> MGAAQSVNGVKIVTNAYAEIMTDLAVDQDITADQTQVFSIDNVSGDVYVEGTVMTEKLVINLASLMKAVTNQSSQDELIDNIAQQAQAAVSGLNFAQF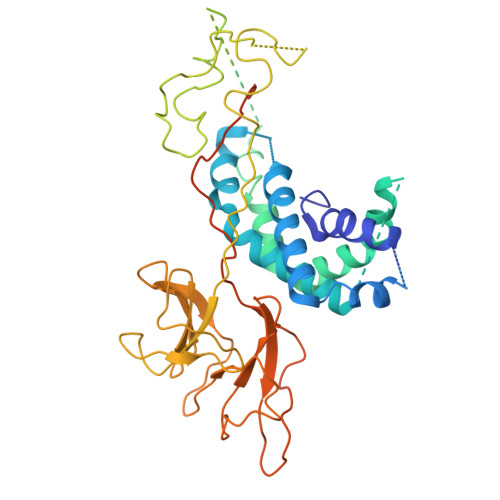AFVTNNIDRLITACVKLSVDMRVSCTAKVEMTQSFSVSSVMGDVRVKDVRMEEFSDVISTCALNAAITNAQLSDIVSQIKQRGDATATGLNPMAILAAVVLAIIGLPLGAGFLAGRRVVGPLMMVTGMVGGGALAMGYVPEPIKLTGFAPEPDLTAVVPVAVENGLTLKAAISKLTGDPQYGAVYWQNYKVTGTTAVKLNQTVSYYAPPNFDPVTWTASEPAQKQPSFRVFPTLFQGQGLPKISYRLAYGTVALTQGPERGDVYLDSTTGNYYVLKDGWKLNGTIPGAIKDRPEAWGIVDPNETTALTGSERYTWVDPYTRVQGTLWYKPKDSHEWVKERQDPVPINVPLTETPSDFNVWVYKDATAKKIVGWVSAGAGAAGAGLTASAYFMPSTAVDAKAEVGEAAK(3R)-3-(dodecanoyloxy)tetradecanoic acid | C26 H50 O4 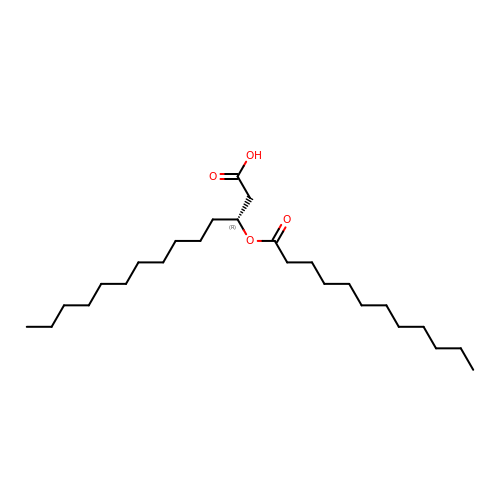| IKRFTYQBIVDIMM-XMMPIXPASA-N>[2x]MHHHHHHTSKIEQPRWASKDS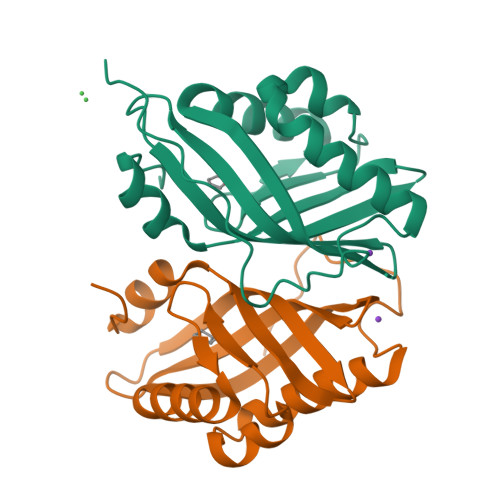AAGAASTPDEKIVLEFMDALTSNDAAKLIEYFAEDTMYQNMPLPPAYGRDAVEQTLAGLFTVMSYDAVETFHIGSSNGLVYTERVDVLRALPTGKSYNVSVLGVFQLTEGKITGWRDYFDLREFEEAVDLPLRG Hepatitis C viruses (HCV) encode a helicase enzyme that is essential for viral replication and assembly (nonstructural protein 3 [NS3]). NS3 contains the typical structural features of a superfamily 2 (SF2) helicase, including the conserved sequence motifs for ATP hydrolysis and RNA recognition. These are arranged within two paradigmatic helicase domains, each of which adopts the RecA fold architecture that is typical for SF2 helicases. Two additional domains contribute to NS3 function, i.e., domain 3, which contains additional motifs for RNA binding and unwinding, and an N-terminally appended protease domain, which enhances helicase activity via a large, positively charged patch that contributes to high-affinity RNA binding.

To carry out the structural studies, we used a conventional “single-chain” construct design in which JFH-1 NS4A amino acids 21 to 34 were fused via a short GSGS linker to the N terminus of JFH-NS3, yielding a full-length NS3 protein in which the β-sheet of the protease domain is stabilized and activated by intercalation of the NS4A fragment. The resulting crystals diffracted to 2.23 Å, in space group P21 21 21, and there is one molecule in the asymmetric unit (ASU). The overall JFH-1 NS3-4A structure is composed of four globular domains arranged in a tetrahedral fashion, as observed previously for gt1b NS3-4A. However, there is a pronounced shift in the position of D2, which is caused by a 9.6° twist in the conserved β14/15 hairpin (amino acids 430 to 452). The twist in the β hairpin propagates into a displacement of D2, altering its position by about 8.7 Å relative to the location of D2 in gt1b structures. Most importantly, the displacement of D2 drives it closer to the protease domain, creating a more narrow, concave area of positively charged residues between D2 and the protease domain. This positive cleft would be expected to improve early, productive contacts with RNA and to confine it in a specific orientation, potentially contributing to the faster and stronger RNA binding by JFH-1 NS3. Similarly, the conserved RNA binding motifs IV (residues 365 to 372) and V (residues 411 to 419) also shift outward by 6.8 Å and 4.2 Å, respectively. Together, these structural differences expand the length of the RNA binding tunnel and would enable JFH-1 NS3 to accommodate one more nucleotide than gt1b NS3, potentially explaining the higher RNA affinity and processivity of the JFH1 variant. In contrast, the RNA binding tunnel in apo-JFH-1 NS3-4A is completely open, resulting in unobstructed access to the RNA binding cleft. The shifted position of D2 prevents the formation of H bonds between Arg393, Gly554, and Glu555 in JFH-1 NS3-4A and frees the cleft to form a known set of interactions with the backbone of single-stranded RNA.

> GCVSIIGRLHVNQRGSGSASITAYAQQTRGLLGAIVVSMTGRDRTEQAGEVQILSTVSQSFLGTTISGVLWTVYHGAGNKTLAGLRGPVTQMYSSAEGDLVGWPSPPGTKSLEPCKCGAVDLYLVTRNADVIPARRRGDKRGALLSPRPISTLKGSSGGPVLCPRGHVVGLFRAAVCSRGVAKSIDFIPVETLDVVTRSPTFSDNSTPPAVPQTYQVGYLHAPTGSGKSTKVPVAYAAQGYKVLVLNPSVAATLGFGAYLSKAHGINPNIRTGVRTVMTGEAITYSTYGKFLADGGCASGAYDIIICDECHAVDATSILGIGTVLDQAETAGVRLTVLATATPPGSVTTPHPDIEEVGLGREGEIPFYGRAIPLSCIKGGRHLIFCHSKKKCDELAAALRGMGLNAVAYYRGLDVSIIPAQGDVVVVATDALMTGYTGDFDSVIDCNVAVTQAVDFSLDPTFTITTQTVPQDAVSRSQRRGRTGRGRQGTYRYVSTGERASGMFDSVVLCECYDAGAAWYDLTPAETTVRLRAYFNTPGLPVCQDHLEFWEAVFTGLTHIDAHFLSQTKQAGENFAYLVAYQATVCARAKAPPPSWDAMWKCLARLKPTLAGPTPLLYRLGPITNEVTLTHPGTKYIATCMQADLEVMT3,6-diamino-1,5-dihydro[1,2,4]triazolo[4,3-b][1,2,4]triazol-4-ium 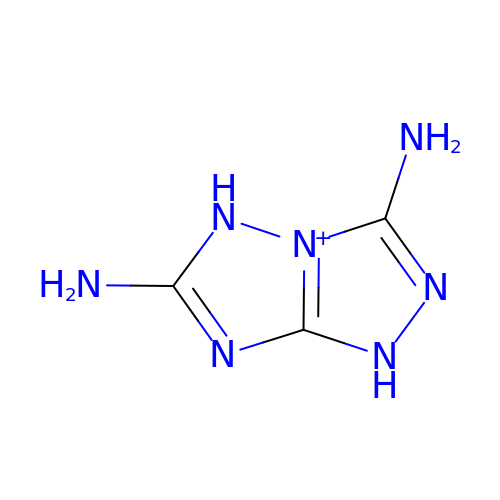| C3 H6 N7 | JFMHNXXJHXPFLE-UHFFFAOYSA-O>MAATTVNGGTVHFKGEVVNAACAVDAGSVDQTVQLGQVRTASLAQEGATSSAVGFNIQLNDCDTNVASKAAVAFLGTAIDAGHTNVLALQSSAAGSATNVGVQILDRTGAALTLDGATFSSETTLNNGTNTIPFQARYFATGAATPGAANADATFKVQYQ[6x];> ADSTITIRGYVRDNGCSVAAESTNFTVDLMENAAKQFNNIGATTPVVPFRILLSPCGNAVSAVKVGFTGVADSHNANLLALENTVSAASGLGIQLLNEQQ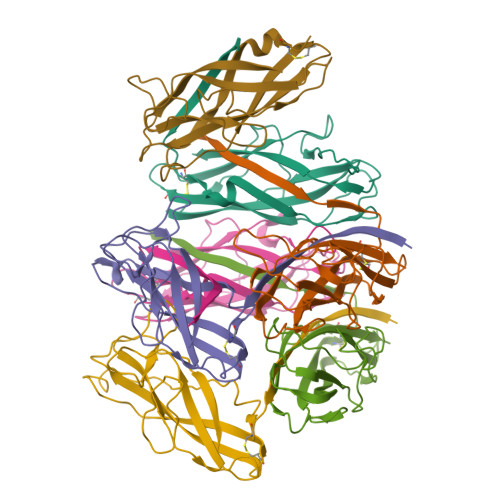NQIPLNAPSSALSWTTLTPGKPNTLNFYARLMATQVPVTAGHINATATFTLEYQ N-(pyridin-2-yl)-2-(1,3,5-trimethyl-1H-pyrazol-4-yl)acetamide | C13 H16 N4 O | 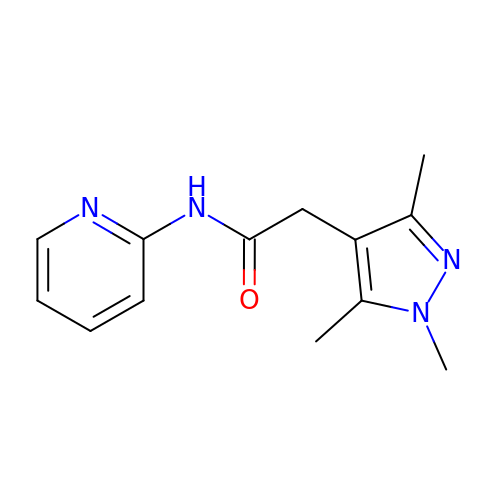OGOQOFZVILXVSY-UHFFFAOYSA-N>[2x]MKSTSDLFNEIIPLGRLIHMVNQKKDRLLNEYLSPLDITAAQFKVLCSIRCAACITPVELKKVLSVDLGALTRMLDRLVCKGWVERLPNPN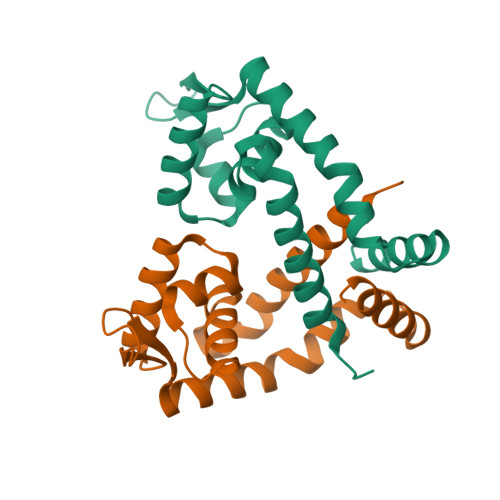DKRGVLVKLTTGGAAICEQCHQLVGQDLHQELTKNLTADEVATLEYLLKKVLP>[2x]MSLISLQSDQLLEATVGQFMIEADKVAHVQVGNNLEHALL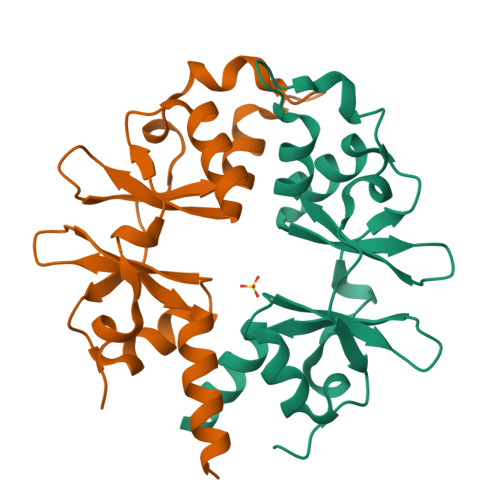VLTKTGYTAIPVLDPSYRLHGLIGTNMIMNSIFGLERIEFEKLDQITVEEVMLTDIPRLHINDPIMKGFGMVINNGFVCVENDEQVFEGIFTRRVVLKELNKHIRSLNKEGGSHHHHHH> LRWQWRIYEEPLQEPLTTAQGVWRSRSGIYLRL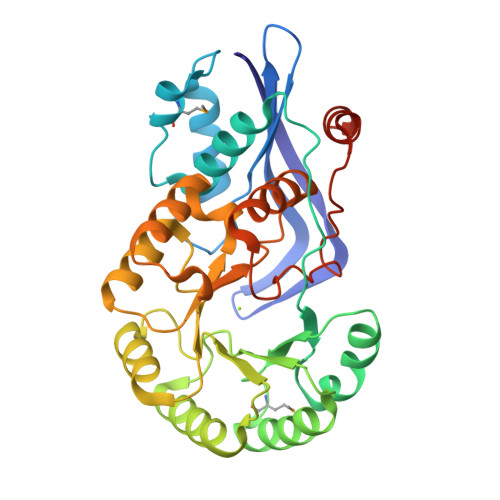EDEQGQVGYGEIAPLPGWGSETLNADIALCQQLPGHLTPEIMATIPEALPAAQFGFATAWQSVGRLPYRVRPWPICALLGSGQAALEQWQQSWQRGQTTFKWKVGVMSPEEEQAILKALLAALPPGAKLRLDANGSWDRATANRWFAWLDRHGNGKIEYVEQPLPPDQWQALLSLAQTVTTAIALDESVVSAAEVQRWVDRGWPGFFVIKTALFGDPDSLSLLLRRGLEPQRLVFSSALEGAIARTAIFHLLETWQPCHALGFGVDRWRSAPLLTTLTAYERLWERLDQEGHHHHHH5-IODODEOXYURIDINE 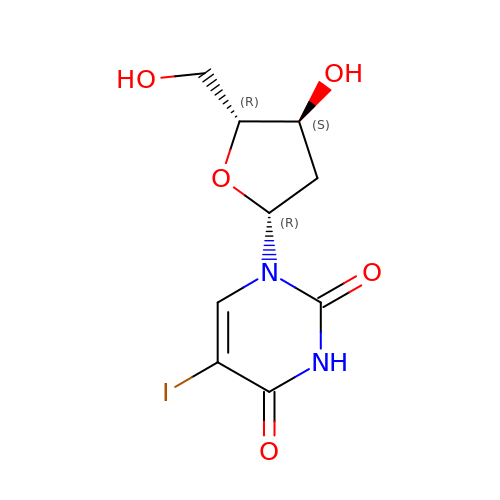| C9 H11 I N2 O5 | XQFRJNBWHJMXHO-RRKCRQDMSA-N>[6x]AIFHTGSELFIITRGPGKLTLLTWGGLNNLRSVIGAIPTENTGVTKWAVSFSHNYTRFSFIWEGQGEACYQIGNGLTRSPVGRSWSSSSTIHWGSSTVITEDVTSVVPGAVNRDKVTTAY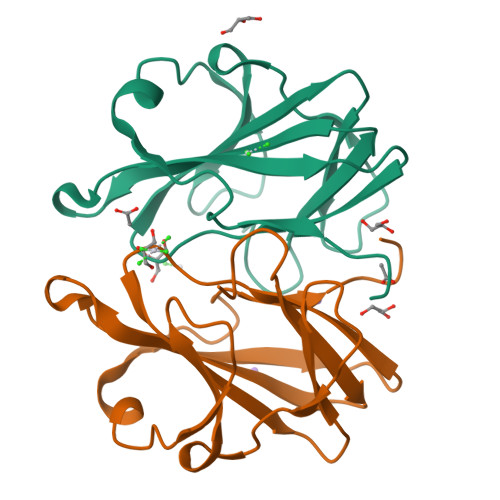ALPDNL5-(4-fluorophenyl)-2,3-dihydroxy-N-(4-thieno[2,3-c]pyridin-2-ylbutyl)benzamide | C24 H21 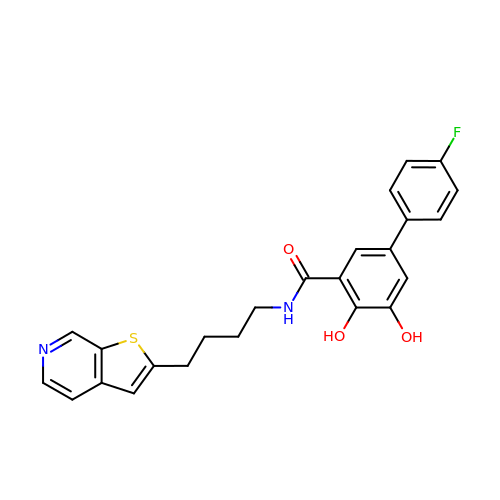F N2 O3 S | XMHHXGQAUPXIKY-UHFFFAOYSA-N>[2x]TPEMPVLENRAAQGDITAPGGARRLTGDQTAALRDSLSDKPAKNIILLIGDGMGDSEITAARNYAEGAGGFFKGIDALPLTGQYTHYALNKKTGKPDYVTDLAASATAWSTGVKTYNGALGVDIHEKDHPTILEMAKAAGLATGNVSTAELQDATPAALVAHVTSRKCYGPSATSEK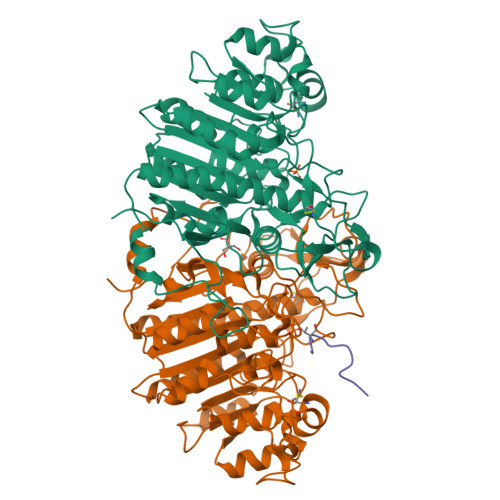CPGNALEKGGKGSITEQLLNARADVTLGGGAKTFAETATAGEWQGKTLREQAQARGYQLVSDAASLNSVTEANQQKPLLGLFADGNMPVRWLGPKATYHGNIDKPAVTCTPNPQRNDSVPTLAQMTDKAIELLSKNEKGFFLQVEGASIDKQDHAANPCGQIGETVDLDEAVQRALEFAKKEGNTLVIVTADHAHASQIVAPDTKAPGLTQALNTKDGAVMVMSYGNSEEDSQEHTGSQLRIAAYGPHAANVVGLTDQTDLFYTMKAALGLKHHHHHH;> HATPPKKEAD> MHHHHHHTTPGEDHAGSFYLPRLEYSTLPMAVDRGVGWKTLRDAGPVVFMNGWYYLTRREDVLAALRNPKVFSSRKALQPPGNPLPVVPLAFDPPEHTRYRRILQPYFSPAALSKALPSLRRHTVAMIDAIAGRGECEAMADLANLFPFQLFLVLYGLPLEDRDRLIGWKDAVIAMSDRPHPTEADVAAARELLEYLTAMVAERRRNPGPDVLSQVQIGEDPLSEIEVLGLSHLLILAGLDTVTAAVGFSLLELARRPQLRAMLRDNPKQIRVFIEEIVRLEPSAPVAPRVTTEPVTVGGMTLPAGSPVRLCMAAVNRDGSDAMSTDELVMDGKVHRHWGFGGGPHRCLGSHLARLELTLLVGEWLNQIPDFELAPDYAPEIRFPSKSFALKNLPLRWS

Ferredoxins are small iron–sulfur proteins and key players in essential metabolic pathways. For catalysis, CYPs required electrons typically supplied by redox proteins, such as ferredoxins. Interestingly, two Mtb 3Fe–4S ferredoxins, Fdx and FdxE, are co-located in respective operons with cytochrome P450 (CYP) enzymes suggesting their functional relevance. Here, we explored the genome context for two ferredoxins, Fdx and FdxE, determined the binding kinetics between FdxE and CYP143, and solved three crystal structures: Fdx, CYP143, and a complex FdxE–CYP143.

To visualize structural changes in CYP143 induced by the interaction with FdxE we solved the CYP143 structure alone at similar resolution (1.4 Å). CYP143 structure is conforming to the typical cytochrome P450 fold with 12 α-helices (A–L) and 4 β-sheets. In the absence of the ligand, protein crystallized in open conformation with the heme cofactor accessible to the bulk solvent. The iron of the heme is hexacoordinated by the invariant Cys342 and a water molecule. This water is stabilized by the H-bond with glycerol molecule from a cryoprotectant solution. Superposition of the CYP143 structure with the CYP143 part of the complex structure shows RMSD = .932Å for all atoms and reveals a different position of the lower part of the meander. In the CYP143 structure alone, the meander is away from the K helix, while in the complex it moves closer and sandwiched between helix 2 of FdxE and K helix of CYP. The relocation distance of 5.5 Å is observed for the Gly327 Ca atom. A closer examination of the interacting regions of CYP143 reveals a different side chain conformation of the charged residues involved in intermolecular contacts with Fdx in a complex structure Gln99 of the C helix, and Arg266 of the K helix. The local proximal area involved in the interaction with FdxE is positively charged, despite overall theoretical pI = 6.8.> MQSWYLLYCKRGQLQRAQEHLERQAVNCLAPMITLEKIVRGKRTAVSEPLFPNYLFVEFDPEVIHTTTINATRGVSHFVRFGASP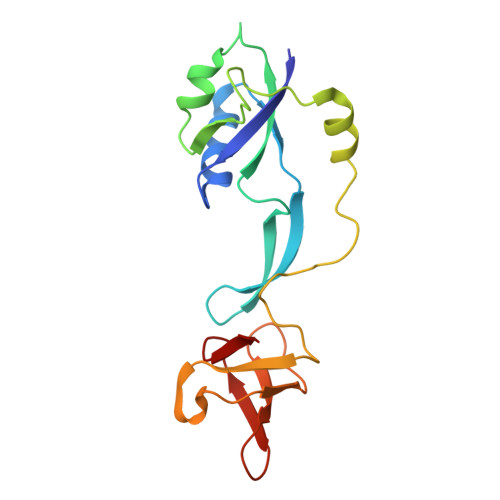AIVPSAVIHQLSVYKPKDIVDPATPYPGDKVIITEGAFEGFQAIFTEPDGEARSMLLLNLINKEIKHSVKNTEFRKL1-[[4-[4-(trifluoromethyl)phenyl]phenyl]methyl]imidazole | C17 H13 F3 N2 | 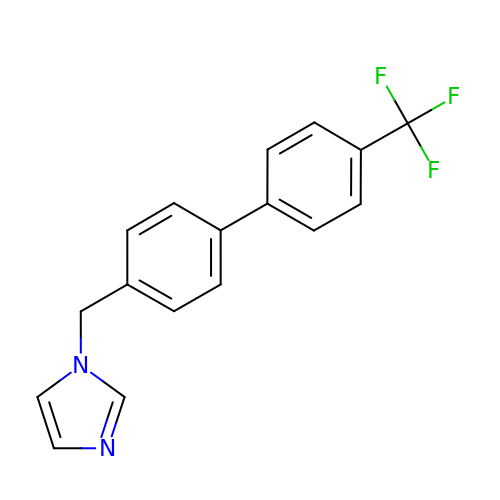ZGVRGKQQDLAUKP-UHFFFAOYSA-N> MELKKMNVPMDTITRDMVRLSEDTENVYETVMIIAKRANQI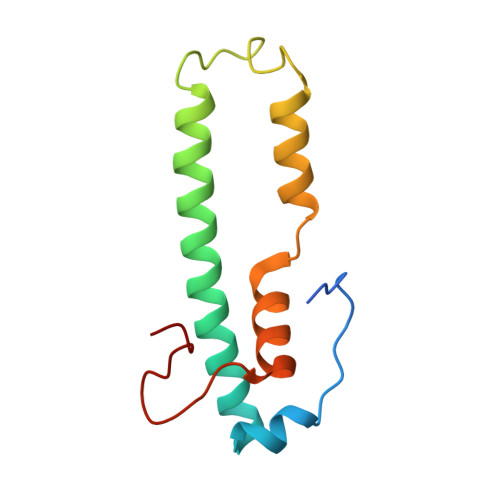GQQMKQDLEKKLQDFSSSNDNLEEVFENREQIEISRYYEHLPKPGLIATAEYEQDKLYHRMPGATSTND> MAKSKRKIDENGYMTIEGCPISSYGVFQYSAGQLGLPGDPMRIVNVYRPESAVSDPEYIESLKNLPLIDEHEMLSGFDDDDDSVAPEDKGVEGIITSNAYYEAPWARGDIRIYSRNMQNQLERGKEDLSLGYSCRYTEQPGIWNGTPYEVVQDKMRGNHIALVKEGRVPGARVLDGLCFDHLSFDFRPSDEGNEMSLKKAKQKPPVQRVGQAADSAVEELRALWPKLSASVQKFLGEEAQEPEHQEGAAAPAEPTDSEHMTEHPTLEGAQKDNEEHEEAPSVVDPAVAAAESERQESAASEMSGEGEVAELISQVKAILARLEGTAAEGADEEHGEGKDVVEGLEEQSSLSGSQTASDDGGEGKDNSEELPEMAQKNAQDAAIRGLYRDIAAKDRLYKRLSSVVGAFDHRAMDSAEVAVYGVKKLNINCAKGQEALALDMYLKGVEASRGAASRQSKAQDSAGSAPQCAELDS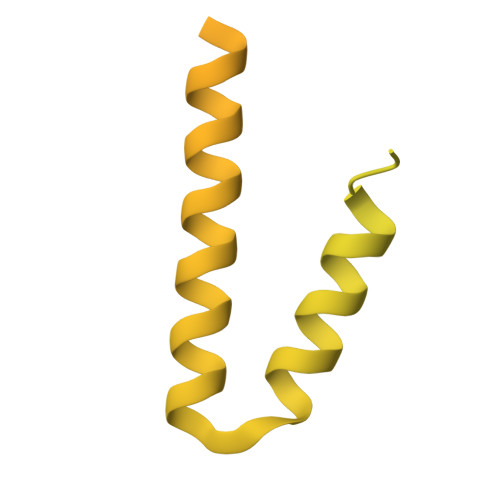YLKGE>[2x]KYRVRKNVLHLTDTEKRDFVRTVLILKEKGIYDRYIAWHGAAGKFHTPPGSDRNAAH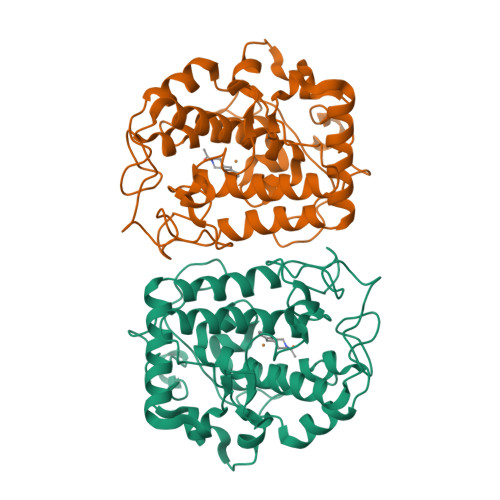MSSAFLPWHREYLLRFERDLQSINPEVTLPYWEWETDAQMQDPSQSQIWSADFMGGNGNPIKDFIVDTGPFAAGRWTTIDEQGNPSGGLKRNFGATKEAPTLPTRDDVLNALKITQYDTPPWDMTSQNSFRNQLEGFINGPQLHNRVHRWVGGQMGVVPTAPNDPVFFLHHANVDRIWAVWQIIHRNQNYQPMKNGPFGQNFRDPMYPWNTTPEDVMNHRKLGYVYDIEL> MSQNNEMHPRNPYRNKPPDFKALAVEYPEFRKFCQYVSNGKVTFDFKKDAAVRCLTQTLLKKDFNLDVEIPPGHLVPRVPQKLNYCLLIDDLLKANKLTKNVIGIDIGTGTSCIHALIGARQFNWKFIATDGDEKSVRVAHENVAKNGLSSSICVVHVNPDVKTVLMDVVNTIPDTDYAFCM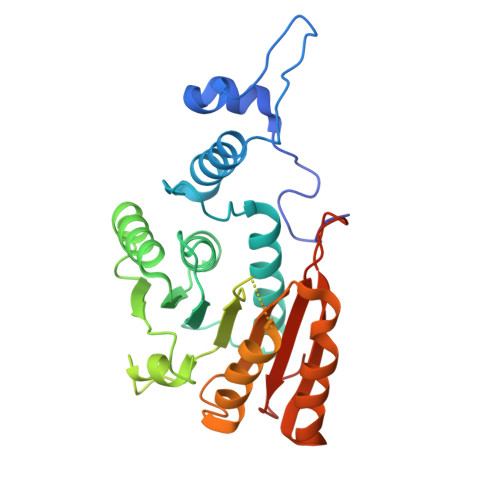CNPPFFEKGNGDDKFCEDISSSTETYSNRVASEFRTAPHSATFASSAELFVDGGEVAFVNRIIDDSVLLRDRIKIYTTMIGRKSSLKPLQNRLQRFGDDVKIMISVLNQGKTKRWMLAWTFSKSVSLTTIDRLEHHHHHH> DDETGKELVLALYDYQEKSPREVTMKKGDILTLLNSTNKDWWK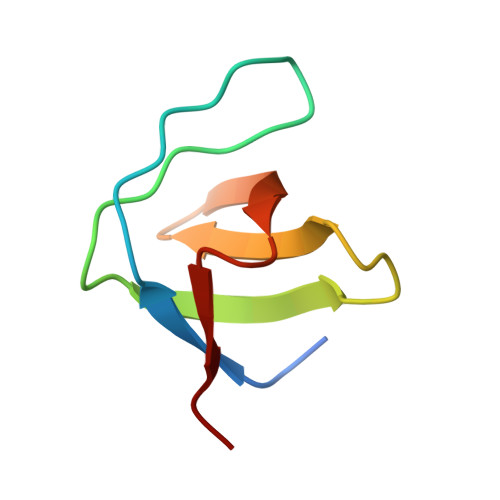VEVADRQGFVPAAYVKKLD> QNWAT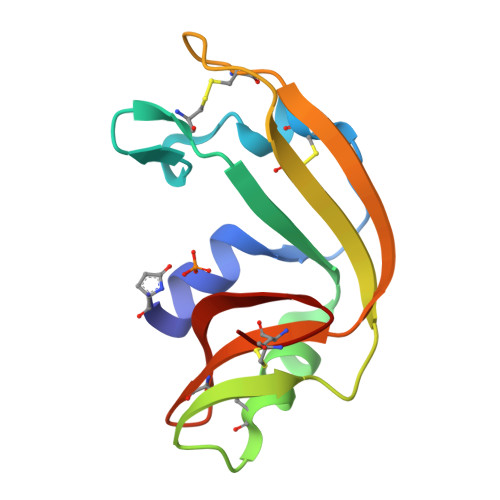FQQKHIINTPIINCNTIMDNNIYIVGGQCKRVNTFIISSATTVKAICTGVINMNVLSTTRFQLNTCTRTSITPRPCPYSSRTETNYICVKCENQYPVHFAGIGRCP> TTDTRRRVKLYALNAERQWDDRGTGHVSSTYVERLKGISLLVRAESDGSLLLESKIQPDT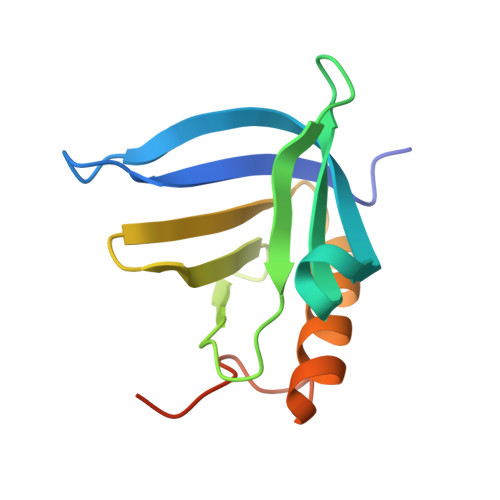AYQKQQDTLIVWSEGDNFDLALSFQEKAGCDEIWEKICQVQGKDPSVEITQDIVEESEDERF>[4x]MKRVVITGLGIVSSIGNNQQEVLASLREGRSGITFSQELKDSGMRSHVWGNVKLDTTGLIDRKVVRFMS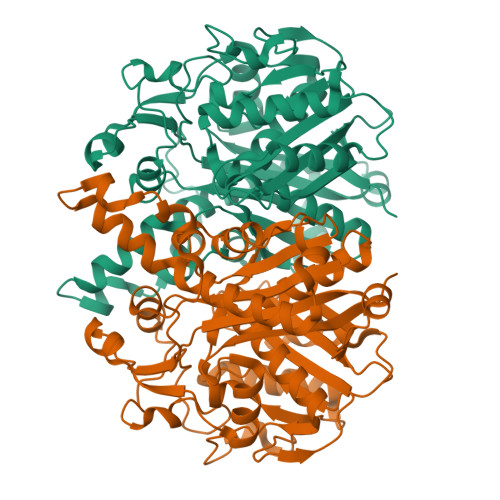DASIYAFLSMEQAIADAGLSPEAYQNNPRVGLIAGSGGGSPRFQVFGADAMRGPRGLKAVGPYVVTKAMASGVSACLATPFKIHGVNYSISSACATSAHCIGNAVEQIQLGKQDIVFAGGGEELCWEMACEFDAMGALSTKYNDTPEKASRTYDAHRDGFVIAGGGGMVVVEELEHALARGAHIYAEIVGYGATSDGADMVAPSGEGAVRCMKMAMHGVDTPIDYLNSHGTSTPVGDVKELAAIREVFGDKSPAISATKAMTGHSLGAAGVQEAIYSLLMLEHGFIAPSINIEELDEQAAGLNIVTETTDRELTTVMSNSFGFGGTNATLVMRKLKD>GAMDPEAAALRAELRDLELEEARLVQELEDVDRNLARAAADL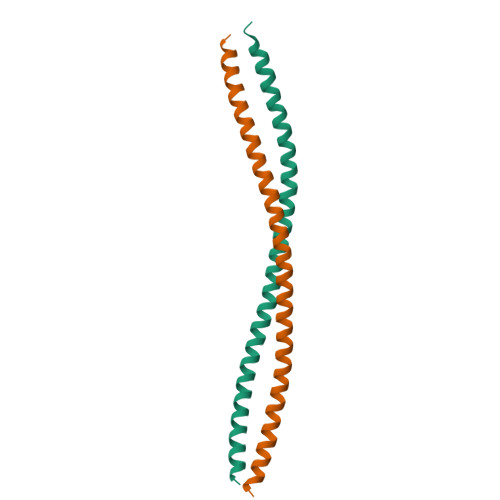QAAQAEAAELDQQERQHYRDYSALKRQQLELLDQLGNVENQLQYARVQRDRLKEIN[4x]> MFKNTFQSGFLSILYSIGSKPLQIWDKSIRNGHIKRITDQDILSSVLEIMGTNVSTNYITAPADPKETLGIKLPFLVMIIKNLKKYYTFEVQVLDDKNVRRRF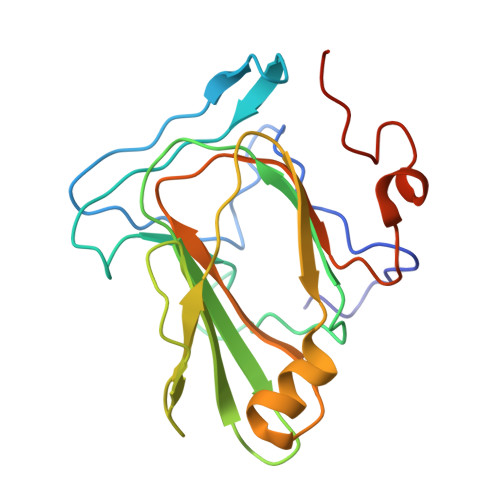RASNYQSTTRVKPFICTMPMRLDEGWNQIQFNLSDFTRRAYATNYIETLRVQIHANCRIRRIYFSDRLYSEEELPPEFKLFLPIQGQNKTNV> MIGIIWDFDGVLVFTPHEKAWKIATEMYGATLTHDFFVKYVSGRPRYEGAANILSRLGIYQKLGVKTEEEKLKLLLEFAELKNRIVNEMFERGEYEVNWE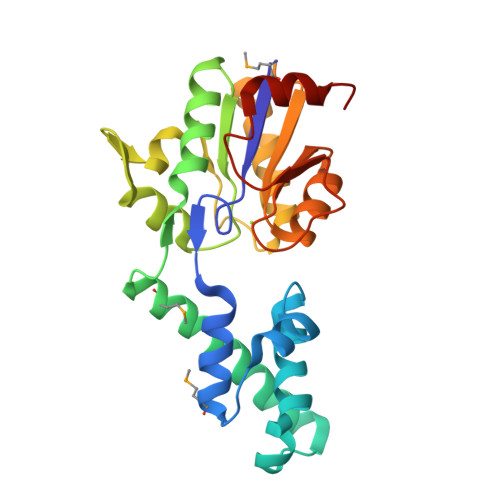AIKFLLETKEKGIKNALASASKNAEKLARKIKVNNKSLLEIFDLNVSGRAETKEDVFKLAKEELKLNFPEIKYFFVVEDAPSGIRAGKAIGAITLGYERESSLEEADFRFSSFGELSVDTLLSLIGGGG> APSYPEYTREEVG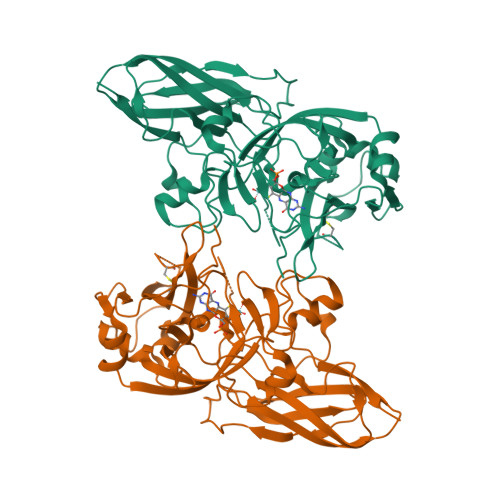RHRSPEERVWVTHGTDVFDVTDFVELHPGGPDKILLAAGGALEPFWALYAVHGEPHVLELLQQYKVGELSPDEAPAAPDAQDPFAGDPPRHPGLRVNSQKPFNAEPPAELLAERFLTPNELFFTRNHLPVPAVEPSSYRLRVDGPGGGTLSLSLAELRSRFPKHEVTATLQSAGNRRSEMSRVRPVKGLPWDIGAISTARWGGARLRDVLLHAGFPEELQGEWHVCFEGLDADPGGAPYGASIPYGRALSPAADVLLAYEMNGTELPRDHGFPVRVVVPGVVGARSVKWLRRVAVSPDESPSHWQQNDYKGFSPCVDWDTVDYRTAPAIQELPVQSAVTQPRPGAAVPPGELTVKGYAWSGGGREVVRVDVSLDGGRTWKVARLMGDKAPPGRAWAWALWELTVPVEAGTELEIVCKAVDSSYNVQPDSVAPIWNLRGVLSTAWHRVRVSVQD>TDIENNVRVVVYIRKDVEDNSQTIEKEGQTVTNNDYHKVYDSLKNMSTVKSVTFSSKEEQYEKLTEIMGDNWKIFEGDANPLYDAYIVEANAPNDVKTIAEDAKKIEGVSEVQD[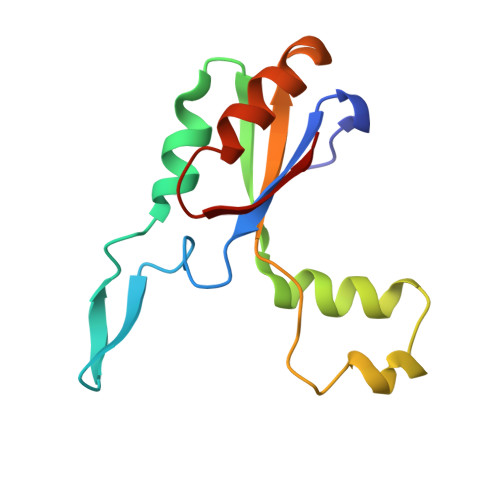2x]>MTISRRDFLNGVALTIAAGLTPAEILRAAPGGRYYPPALTGLRGSHPGAFEVAHQMGWEKKTFDVDHLPIEEEYDLVVVGGGISGLAAAWFYRERHPAARILVIENHDDFGGHAKRNEFQAGGRTILGYGGSESLQSPNALYSEDAKHLLKRLGVELKRFETA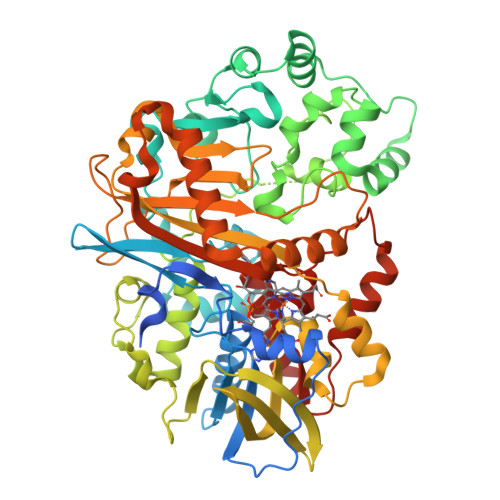FDTDFYPGLGLSRAVFFDKASFGVDKLVSGDPTPMVADEVPRDRLNARSWRAFIGDFPLSREDREALIALYESPRDYLAGKSVEEKETYLAKTSYRDYLLKNVGLSETSVKYFQGRSNAFSALGADALPAADAYAAGFPGFDALGLPQPSEEAQAEMDEPYIYHFPDGNASLARLMVRDLIPAVAPGRGMEDIVMARFDYSKLDLAGHPVRLRLNSTAVSVRNRAGGVDVGYSRAGRLHRVRGKHCVMACYNMMVPYLLRDLSEEQAHALSQNVKFPLVYTKVLLRNWQAWKTLGIHEIYAPTLPYSRIKLDFPVDLGSYRHPRDPRQPIGVHMVYVPTTPNAGMDARTQARVGRSKLYAMSFEQLEKDIRDQLQAMLGPAGFDHRRDITGITVNRWSHGYSYFMNTLYDDEAESEALMELARSKVGNVAIANSDAAWDAYAHAAIDQAVRAVRELG[2x]> MQSGLCHCVRRVAALGSVANLHHFTNLPSGFSVWTSRRWQSQSSRGQPGLQWQEGVVDPRYSSSGNMRRFNPDTVAHYVKATIQNDRREMGLGEVYDWHEFAKDAVYIPTRSGPLWVGSDDPRCAKFMRRRSKMQKTPQQKARPKPGPDPAKALEDHPLREYFTTATNLRDPLSTANNLHRAGLIREYDIKYTAAKVRYVPRPPVVSIMGHVDHGKTTLLDYLRKTNVASQEAGGITQNVGAFQVKTLGDTLVTFIDTPGHAAFTTMREVGATANDLIVLVVSAVDGVQPQTKEVIELAHKSGIPFV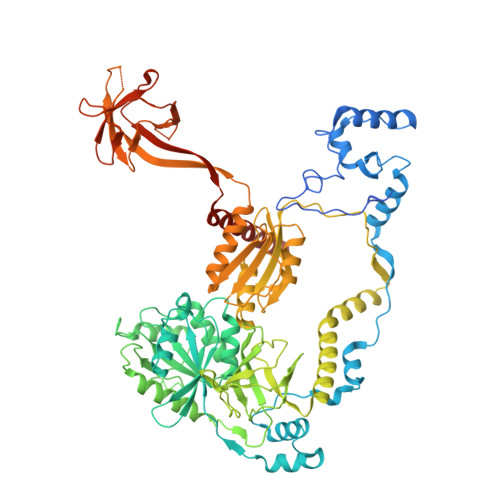VACTKIDRQPRVENVKQQLRDCNVELEEDGGDTQFVPVCARDGRGVPELLEAIALQAELCEISTPKPSRCEVTVIETNGVNTTTEVAGIVRCGKVRAGQVLVAGMTYAVVRKVLDEHGQIIQEAGPSQPVVLHGFRVHPKPGSILLQVSSESHAQKFYHFMKEVYQAEGRREDYLQLLNQEQHGMLYARKPDNNLVRTYSTQAFVLSCKAATFGMLQALMKSIYEIPRLEGISTEIKVTEVGGLRDYDVALIGSSGQPGCILLYGGCKDTNTLDVPNHVTVIRFNVLYHGLEALKETLVGALPKITKIRVTAEAECLQVFRASQAGKSGNAGGMRVTKGTIIAAHLTFRVCRKAPLVKGTAETDGVSDNEGDGDEDMLGHRVVVYEGQIKELRRFKELVPSVELGLECGVIMQDEFQFRTGDILQQYETYEEPRDVAEEYQKAELREKIMRDTAAAEALLAESTGGEDKPTEESEVKTTI> MTTRPAESAPQTASTLLEPGSNGVVRLLGGPGTGKSSLLVDTAVQHILAGADPESVLLLTGSARLRTAARAAITARLLGAGTVGVVREPLVRTVHSYAFAVLRLAAQRNGDPPPRLITSAEQDGIIRELLAGDLEDGHRSPVGWPEQLWPALTTAGFATELRDLMARCTERGVDPIALQRLGRTAKRPEWLAAGRFAQAYEQIMLLRSAVGMAAPQATVPALGAAELVGAALEALGADDELLDTERNRIKLLLVDDAQHLDPQAARLVRALAAGTGLTVIAGDPDQSVFGYRGADPVLLRDDTHPAITLTQSYRCAPEIASAITGLGQRLPGVSDTRHWTGNPQREGTVTVRLAASTHAEGTMIADALRRAHLVDGIPWSQMAVIVRSVPRVGTALARALTAAGVPVQDNGTDVPVGRQPAAAALLTVLDVTATGHLDADSAVALLTGPIGRVDPVTLRQLRRALRRADGSQPPRDFGDLLVDAIEREPKGLSAEHARTLRRLRAVLTAARRSDASGADPRYTLWQAWHASGLQRRWLAASERGGSVGAQADRDLDAVTTLFDVADQYVNRTAGASLRGLVDHVTRLGAAVARTEPETAAEAVAVLSVHGALAGEWDFVVIAGVQEGLWPNMIPRGGVLGTQHLVDVLDG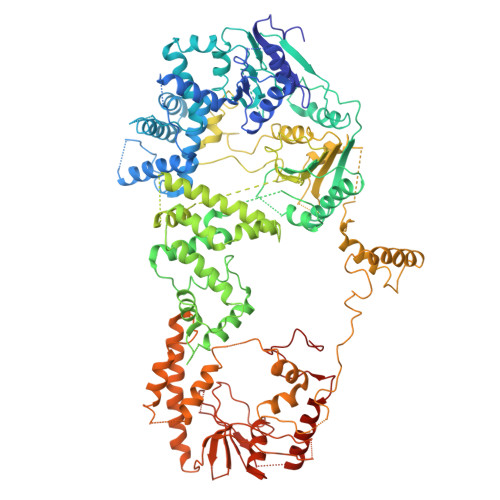VADMTDRTVSTRAPLVAEERRLLMAAMGRARTRVMITAVDSDTGDESLLPSPFCAEISAWATEPVAEPPLVAPRVLAPSALVGRLRAVVCAPDGAVDDDARACAAAQLARLAAAGVPGADPSQWHAMTSLTTEEPLWSEPGHVVTLSPSTLQMLTDCPLRWLLERHGGDDGRDVRSTVGSLVHALVSEPGKTESQLVNELEKVWDDLPYDAKWYSDNELARHRAMLETFTRWREDTRRQLTEVATEIPVEGIVVEPGENTPGVRVRGRLDRLERDEAGRLVVVALKTGKSPVTKDDAQNHAQLAMYQLAVAAGLLDDGDEPGGGKLVYLGKAGAAGATEREQDPLTPDKRAEWLETVGEAAAATAGPRFVARVNNGCANCPVRSSCPAQANGDRP>[2x]MEKVREIVREGIRVGNEDPRRIIHAFKVGLALVLVSSFYYYQPFGPFTDYFGINAMWAVMTVVVVFEFSVGATLGKGLNRGVATLVAGGLGIGAHQLARLSGATVEPI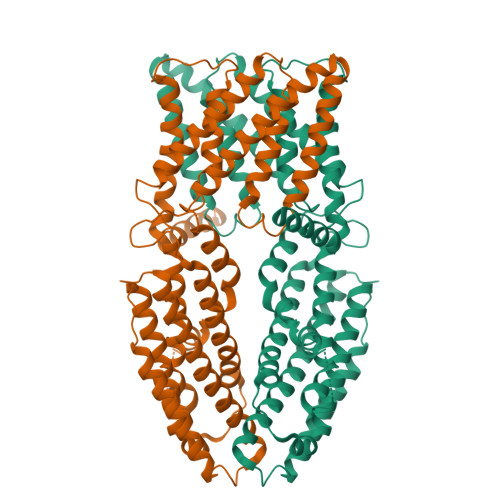LLVMLVFVQAALSTFVRFFPWVKTKFDYGILIFILTFALISLSGFRDEEIMDLAESRLSTVVIGGVSCILISIFVCPVWAGQDLHSLLASNFDTLSHFLQDFGDEYFEAREKGDYKVVEKRKKNLERYKSVLDSKSDEEALANYAEWEPPHGQFRFRHPWKQYVAVGALLRQCAYRIDALNSYINSDFQIPVDIKKKLETPLRRMSSESGNSMKEMSISLKQMIKSSSSDIHVSNSQAACKSLSTLLKSGILNDVEPLQMISLMTTVSMLIDIVNLTEKISESVHELASAARFKNKMRPTVLYEKSDSGSIGRAMPIDSHEDHHVVTVLHDVDNDRSNNVDDSRGGSSQDSCHHVAIKIVDDNSNHEKHEDGEIHVHTLSNGHLQ> SMDYQLVQHEVLCSMTNTYEVLEFLGRGTFGQVVKCWKRGTNEIVAIKILKNHPSYARQGQIEVSILARLSTESADDYNFVRAYECFQHKNHTCLVFEMLEQNLYDFLKQNKFSPLPLKYIRPVLQQVATALMKLKSLGLIHADLKPENIMLVDPSRQPYRVKVIDFGSASHVSKAVCSTYLQSRYYRAPEIILGLPFCEAIDMWSLGCVIAELFLGWPLYPGASEYDQIRYISQTQGLPAEYLLSAGTKTTRFFNRDTD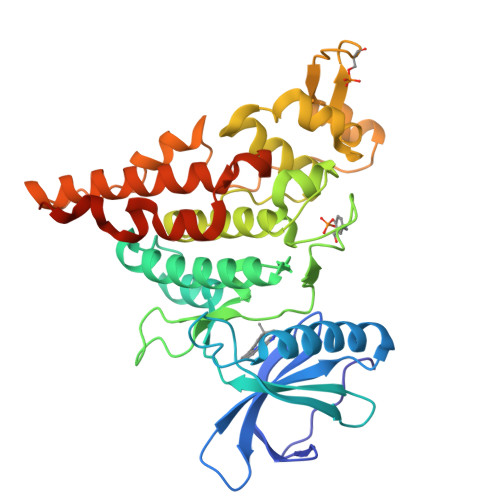SPYPLWRLKTPDDHEAETGIKSKEARKYIFNCLDDMAQVNMTTDLEGSDMLVEKADRREFIDLLKKMLTIDADKRITPIETLNHPFVTMTHLLDFPHSTHVKSCFQN>[2x]MEAVVISGRKLAQQIKQEVRQEVEEWVASGNKRPHLSVILVGENPASHSYVLNKTRAAAVVGINSETIMKPASISE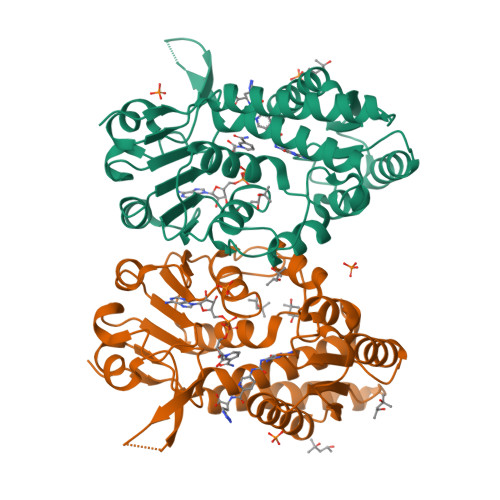EELLNLINKLNNDDNVDGLLVQLPLPEHIDERRICNAVSPDKDVDGFHVINVGRMCLDQYSMLPATPWGVWEIIKRTGIPTLGKNVVVAGRSKNVGMPIAMLLHTDGAHERPGGDATVTISHRYTPKEQLKKHTILADIVISAAGIPNLITADMIKEGAAVIDVGINRVHDPVTAKPKLVGDVDFEGVRQKAGYITPVPGGVGPMTVAMLMKNTIIAAKKVLRLEEREVLKSKELGVATN> AASEETLAFQRQLNALIGYDVTDVSNVHDDELEFTRRRLVTPRMAEVAGRDPKLYAMHPWVTSKPLPEYLLKKITNNCVFIVIHRSTTSQTIKVSADDTPGTILQSFFTKMAKKKSLMDIPESQNERDFV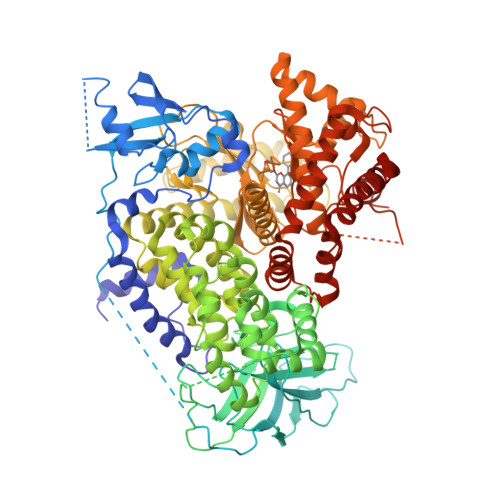LRVCGRDEYLVGETPIKNFQWVRQCLKNGEEIHLVLDTPPDPALDEVRKEEWPLVDDCTGVTGYHEQLTIHGKDHESVFTVSLWDCDRKFRVKIRGIDIPVLPRTADLTVFVEANIQYGQQVLCQRRTSPKPFTEEVLWNVWLEFSIKIKDLPKGALLNLQIYCGKAPALSGKTSAEMPSPESKGKAQLLYYVNLLLIDHRFLLRHGEYVLHMWQLSGKGEDQGSFNADKLTSATNPDKENSMSISILLDNYCHPIALPKHRPTPDPEGDRVRAEMPNQLRKQLEAIIATDPLNPLTAEDKELLWHFRYESLKDPKAYPKLFSSVKWGQQEIVAKTYQLLAKREVWDQSALDVGLTMQLLDCNFSDENVRAIAVQKLESLEDDDVLHYLLQLVQAVKFEPYHDSALARFLLKRGLRNKRIGHFLFWFLRSEIAQSRHYQQRFAVILEAYLRGCGTAMLHDFTQQVQVIDMLQKVTIDIKSLSAEKYDVSSQVISQLKQKLENLQNLNLPQSFRVPYDPGLKAGALVIEKCKVMASKKKPLWLEFKCADPTALSNETIGIIFKHGDDLRQDMLILQILRIMESIWETESLDLCLLPYGCISTGDKIGMIEIVKDATTIAKIQQSTVGNTGAFKDEVLSHWLKEKCPIEEKFQAAVERFVYSCAGYCVATFVLGIGDRHNDNIMISETGNLFHIDFGHILGNYKSFLGINKERVPFVLTPDFLFVMGTSGKKTSLHFQKFQDVCVKAYLALRHHTNLLIILFSMMLMTGMPQLTSKEDIEYIRDALTVGKSEEDAKKYFLDQIEVCRDKGWTVQFNWFLHLVLGIKQGEKHSA> MTEQRPLTIALVAGETSGDILGAGLIRALKEHVPNARFVGVAGPRMQAEGCEAWYEMEELAVMGISESSGRSRRSSHIRADLTKRFGELKPDVFVGIDAPDFNITLEGNLKKQGIKTIHYVSPSVWAWRQKRVFKIGRATDLVLAFLPFEKAFYDKYNVPCRFIGHTMADAMPLDPDKNAARDVLGIPHDAHCLALLPGSRGAEVEMLSADFLKTAQLLRQTYPDLEIVVPLVNAKRREQFERIKAEVAPDLSVHLLDGMGREAMVASDAALLASGTAALECMLSKCPMVVGYRMKPFTFWLAKRLVKTDYVSLPNLLAGRELVKELLQEECEPQKLAAALLPLLANGKTSHAMHDTFRELHQQIRCNADEQAAQAVLELAQ

During LPS biosynthesis, a membrane-associated glycosyltransferase (LpxB) forms a tetra-acylated disaccharide that is further acylated to form the membrane anchor moiety of LPS. LpxB is a glycosyltransferase in the Raetz (lipid A synthesis) pathway that catalyzes nucleophilic attack of the 6′-hydroxyl of lipid X (1) on the anomeric carbon of UDP-diacyl-glucosamine (UDP-DAG) (2) to form β(1–6)-tetraacyl-disaccharide 1-phosphate (lipid A disaccharide) (3). Here we present the first crystal structures of a soluble variant of E. coli LpxB in the apo form and bound to UDP, which reveals a novel glycosyltransferase-B (GT-B) dimer wherein the C-terminal tail of one subunit completes the fold of the other subunit. The structure reveals that LpxB has a glycosyltransferase-B family fold but with a highly intertwined, C-terminally swapped dimer comprising four domains.

In order to crystallize LpxB, a soluble form of the enzyme was generated. We identified, and mutated to Ser, six Val and Leu residues (V66, V68, L69, L72, L75, and L76) in a nearby region of the LpxB homology model. These mutations improved solubility and yield of LpxB, and the LpxB with all six mutations (LpxB6S) showed the least aggregation on a size exclusion column. LpxB6S was used for initial crystallization screening and optimization. LpxB6S was crystallized with one molecule in the asymmetric unit. However, the biological assembly is a highly intertwined, C-terminally swapped homodimer. In vitro activity assays suggested that the ability of LpxB6S to catalyze the reaction of Triton X-100-solubilized substrates was completely abolished. However, when the substrates were solubilized with 0.9 M 3-(1-Pyridinio)-1-propanesulfonate (NDSB 201), residual lipid A disaccharide synthesis was observable for LpxB6S by thin layer chromatography (TLC), but LpxB6S activity remained below the detection limit for UDP-release assays even with the addition of NDSB 201. These results demonstrate that LpxB6S remains catalytically competent and suggest that this solubilized form of the enzyme fails to extract lipid substrates from detergent micelles. In contrast, the knockout was not obtained when the gene for LpxB6S, LpxB6S-R201A, or LpxBR201A was substituted on the plasmid. These results suggest that the hydrophobic patch (V66, V68, L69, L72, L75, and L76) is essential for productive membrane association or substrate binding.>MSYCRQEGKDRIIFVTKEDHETPSSAELVADDPNDPYEEHGLILPNGNINWNSPSLGGMASGPCGEQFKSAFSCFHYSTEEIKGSDCVDQFRAMQECMQKYPDLYPQEDEDEEEEREKKPAEQAEETAPIEATATKEEEGSSLEHHHHHH[2x];>MASMTGGQQMGRGSEFMGGLTPEQKQKKAALSASEGEEVPQDKAPSHVPFLLIGGGTAAFAAARSIRARDPGARVLIVSEDPELPYMRPPLSKELWFSDDPNVTKTLRFKQWNGKERSIYFQPPSFYVSAQDLPHIENGGVAVLTGKKVVQLDVRDNMVKLNDGSQITYEKCLIATGGTPRSLSAIDRAGAEVKSRTTLFRKIGDFRSLEKISREVKSITIIGGGFLGSELACALGRKARALGTEVIQLFPEKGNMGKILPEYLSNWTMEKVRREGVKVMPNAIVQSVGVSSGKLLIKLKDGRKVETDHIVAAVGLEPNVELAKTGGLEIDSDFGGFRVNAELQARSNIWVAGDAACFYDIKLGRRRVEHHDHAVVSGRLAGENMTGAAKPYWHQSMFWSDLGPDVGYEAIGLVDSSLPTVGVFAKATAQDNPKSATEQSGTGIRSESETESEASEITIPPSTPAVPQAPVQGEDYGKGVIFYLRDKVVVGIVLWNIFNRMPIARKIIKDGEQHEDLNEVAKLFNIHEDAAALEHHHHHH[2x]

Apoptosis-inducing factor mitochondrial 1 (AIFM1) is a NADH-binding flavin adenine dinucleotide (FAD)-dependent oxidoreductase in the mitochondrial intermembrane space (IMS). It plays key roles in mitochondrial function, respiratory chain maintenance, redox control, and non-caspase-dependent cell death. Upon NADH binding, an air-stable FADH2-NAD+ charge-transfer complex (CTC) forms, inducing AIFM1 dimerization and the release of a C-terminal regulatory segment termed C-loop. We solved three structures of human soluble AIFM1 (aa 103–613) by cryo-EM: the dimer (1) without interactors (termed “AIFM1 dimer”), (2) bound to AK2A, or (3) to MIA40.

The unstructured N-terminal region of MIA40 mediates the interaction with AIFM1.13,15 A recent crystal structure revealed the interaction of a MIA40 β-hairpin (amino acids, aa 3–15) with the AIFM1 C-terminal region (aa 491–510 and 562–611) by parallel β-strand complementation. We obtained reconstructions for the AIFM1 dimer and AIFM1-AK2A and AIFM-MIA40 complexes at global resolutions of 2.8, 2.6, and 2.4 Å, respectively. AK2A and MIA40 bind the same β-sheet of the AIFM1 C-terminal domain (aa 480–510 and 559–580) via parallel β-strand complementation, adding one and two β-strands, respectively. MIA40 Y3 stacks with F14 to stabilize the second β-strand. MIA40, however, induced up to 3 Å Cα RMSD (root-mean-square deviation) variability compared with the AIFM1 dimer, particularly of the NAD-binding domain, with the strongest displacement of the α-helix contacting the C-terminal domain (aa 345–359). The NAD-binding domain shifts toward the N-terminal domain and dimer interface, also reflected in the relative position of the NAD and FAD cofactors upon MIA40 binding. However, in AIFM1-MIA40, the distance between the nicotinamide and isoalloxazine rings is reduced by approx. 0.2 Å. Despite uncertainties in the side chain densities of K177 (probably flexible) and E314 (degraded by beam-induced damage), our AIFM1-MIA40 map suggests distinct conformations of E314 and K177 in the AIFM1 protomers of AIFM1-MIA40: one resembles the AIFM1 dimer and AIFM1-AK2A structures, whereas the other K177 side chain points away from the cofactors, releasing interactions with E314 and the FAD isoalloxazine. MIA40 adds two β-strands and leads to a compaction of AIFM1, in particular the NAD-binding domain, leading to a compacted active site and shorter distance between the nicotinamide of NAD and the isoalloxazine of FAD. The MIA40 peptide decreased the apparent KM and increased kcat (0.09 mM, 0.89 s−1), indicating increased AIFM1 redox activity even at physiological concentrations of NADH (5–160 μM, total cytosolic NAD between 50 and 500 μM).>MKLNFSGLRALVTGAGKGIGRDTVKALHASGAKVVAVTRTNSDLVSLAKECPGIEPVCVDLGDWDATEKALGGIGPVDLLVNNAALVIMQPFLEVTKEAFDRSFSVNLRSVFQVSQMVARDMINRGVPGSIVNVSSMVAHVTFPNLITYSSTKGAMTMLTKAMAMELGPHKIRVNSVNPTVVLTDMGKKVSADPEFARKLKERHPLRKFAEVEDVVNSILFLLSDRSASTS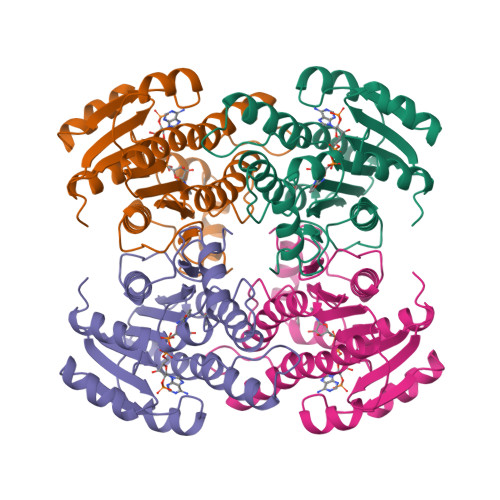GGGILVDAGYLAS[4x]> QCDNFPQMLRDLRDAFSRVKTFFQTKDEVDNLLLKESLLEDFKGYLGCQALSEMIQFYLEEVMPQAENQDPEAKDHVNSLGENLKTLRLRLRRCHRFLPCENKSKAVEQIKNAFNKLQEKGIYKAMSEFDIFINYIEAYMTIKAR;> HGTELPSPPSVWFEAEFFHHILHWTPI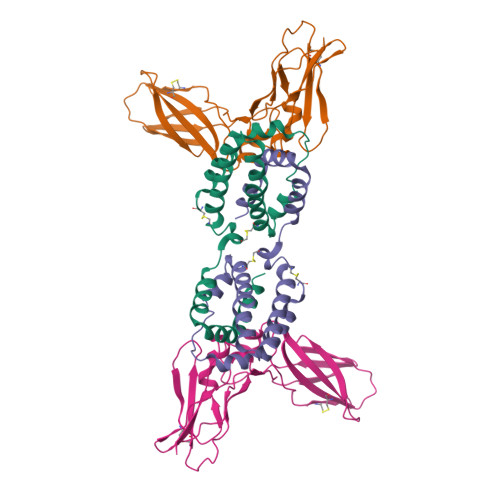PQQSESTCYEVALLRYGIESWNSISQCSQTLSYDLTAVTLDLYHSNGYRARVRAVDGSRHSQWTVTNTRFSVDEVTLTVGSVNLEIHNGFILGKIQLPRPKMAPAQDTYESIFSHFREYEIAIRKVPGQFTFTHKKVKHEQFSLLTSGEVGEFCVQVKPSVASRSNKGMWSKEECISLTRQYFTVTN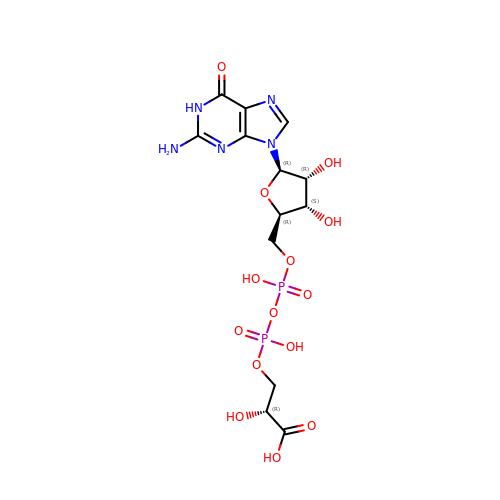3-(guanosine-5'-diphospho)-D-glycerate | C13 H19 N5 O14 P2 | UBONPDGCIQEDRL-QWEIRQIHSA-N>GEPRTKRQAISAEPTAFDIQDLSHVTLPFYPKSPQSKDLIKEAILDNDFMKNLELSQIQEIVDCMYPVEYGKDSCIIKEGDVGSLVYVMEDGKVEVTKEGVKLCTMGPGKVFGELAILYNCTRTATVKTLVNVKLWAIDRQCFQTIMMRTGLIKHTEYMEFLKSVPTFQSLPEEILSKLADVLEETHYENGEYIIRQGARGDTFFIISKGTVNVTREDSPSEDPVFLRTLGKGDWFGEKALQGEDVRTANVIAAEAVTCLVIDRDSFKHLIGGLDDVSNKAYEDAEAKAKYEAEAAFFANLKLSDFNIIDTLGVGGFGRVELVQLKSEESKTFAMKILKKRHIVDTRQQEHIRSEKQIMQGAHSDF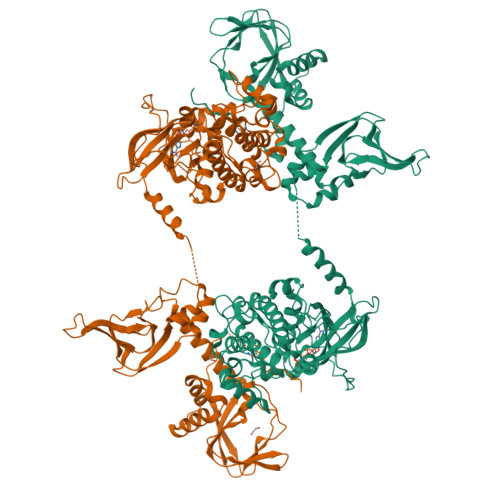IVRLYRTFKDSKYLYMLMEACLGGELWTILRDRGSFEDSTTRFYTACVVEAFAYLHSKGIIYRDLKPENLILDHRGYAKLVDFGFAKKIGFGKKTWTFCGTPEYVAPEIILNKGHDISADYWSLGILMYELLTGSPPFSGPDPMKTYNIILRGIDMIEFPKKIAKNAANLIKKLCRDNPSERLGNLKNGVKDIQKHKWFEGFNWEGLRKGTLTPPIIPSVASPTDTSNFDSFPEDNDEPPPDDNSGWDIDF[2x]>MRCIGISNRDFVEGVSGGSWVDIVLEHGSCVTTMAKNKPTLDFELIKTEAKQPATLRKYCIEAKLTNTTTDSRCPTQGEPSLNEEQDKRFVCKHSMVDRGWGNGCGLFGKGGIVTCAMFTCKKNMKGKVVQPENLEYTIVITPHSGEEHAVGNDTGKHGKEIKITPQSSITEAELTGYGTVTMECSPRTGLDFNEMVLLQMENKAWLVHRQWFLDLPLPWLPGADTQGSNWIQKETLVTFKNPHAKKQDVVVLGSQEGAMHTALTGATEIQMSSGNLLFTGHLKCRLRMDKLQLKGMSYSMCTGKFKVVKEIAETQHGTIVIRVQYEGDGSPCKIPFEIMDLEKRHVLGRLITVNPIVTEKDSPVNIEAEPPFGDSYIIIGVEPGQLKLNWFKKGSSIGQMIETTMRGAKRMAILGDTAWDFGSLGGVFTSIGKALHQVFGAIYGAAFSGVSWIMKILIGVIITWIGMNSRSTSLSVSLVLVGVVTLYLGVMVQA[3x];>[3x]FHLTTRNGEPHMIVSRQEKGKSLLFKTEDGVNMCTL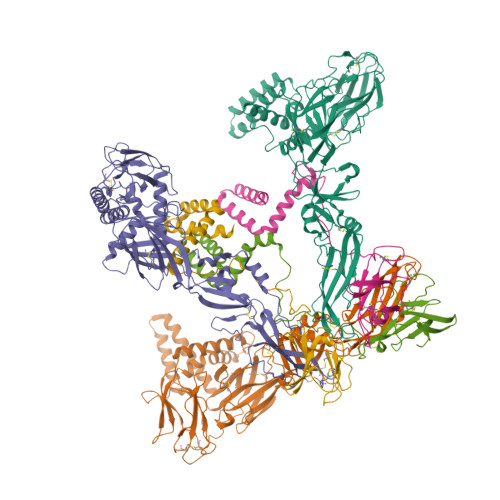MAMDLGELCEDTITYKCPFLKQNEPEDIDCWCNSTSTWVTYGTCTTTGEHRREKRSVALVPHVGMGLETRTETWMSSEGAWKHAQRIETWILRHPGFTIMAAILAYTIGTTHFQRALIFILLTAVAPSMT> CHLSDMLQQLHSVNASKPSERGLVRQEEAEDPACIPIFWVSKWVDYSDKYGLGYQLCDNSVGVLFNDSTRLILYNDGDSLQYIERDGTESYLTVSSHPNSLMKKITLLKYFRNYMSEHLLKAGANITPREGDELARLPYLRTWFRTRSAIILHLSNGSVQINFFQDHTKLILCPLMAAVTYIDEKRDFRTYRL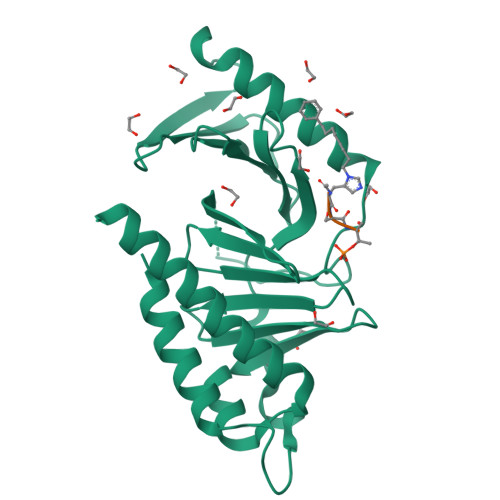SLLEEYGCCKELASRLRYARTMVDKLLSSRSASNR>[2x]GAMGFNKILVVCVGNICRSPTG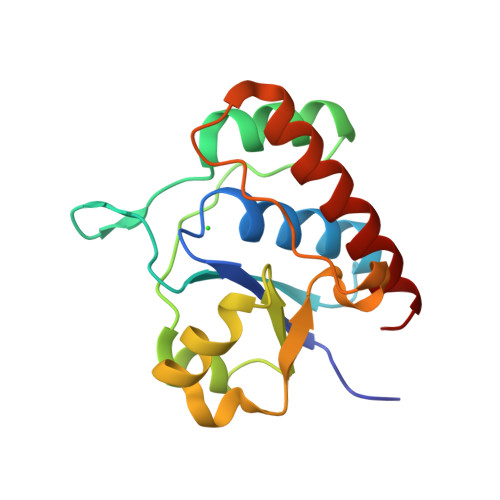ERVLQKLLPNKTVASAGIAAEKSRLIGKPADAMAIEVAKENCVDVENHQSQQLTSALCSQYDLILVMEKGHMEALTQIAPEARGKTMLFGQWIGQKDIPDPYRQSKEAFVHAYQLIDEAAQAWAKKL>[4x]MSGTLYIVSAPSGAGKTSLVKALLDAAPEVRVSVSHTTRGMRPGEVDGVNYHFTSREEFLA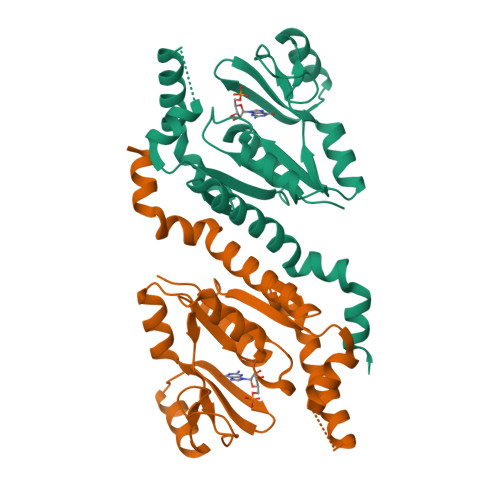MLERNEFLEHAEVFGNLYGTSQRWVEKTLAEGLDLILEIDWQGAQQVRRLMPEAQSIFILPPSQEALRQRLTNRGQDSDEVIERRMREAVSEMSHYVEYDHLVINDDFAHALDDLKAIFRARQLRQDAQQQRHAELLGRLLAGHHHHHH>[2x]MEFTTGLMSLDTALNEMLSRVTPLTAQETLPLVQCFGRI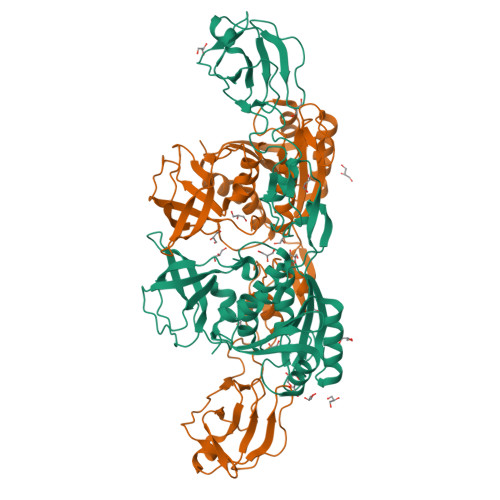LASDVVSPLDVPGFDNSAMDGYAVRLADIASGQPLPVAGKSFAGQPYHGEWPAGTCIRIMTGAPVPEGCEAVVMQEQTEQMDNGVRFTAEVRSGQNIRRRGENISAGAVVFPAGTRLTTAELPVIASLGIAEVPVIRKVRVALFSTGDELQLPGQPLGDGQIYDTNRLAVHLMLEQLGCEVINLGIIRDDPHALRAAFIEADSQADVVISSGGVSVGEADYTKTILEELGEIAFWKLAIKPGKPFAFGKLSNSWFCGLPGNPVSATLTFYQLVQPLLAKLSGNTASGLPARQRVRTASRLKKTPGRLDFQRGVLQRNADGELEVTTTGHQGSHIFSSFSLGNCFIVLERDRGNVEVGEWVEVEPFNALFGGL>KDYPDNVMTAEMRKIAMAAVLSGMRVNMCASPASSPNVIWAIELEAEGSGSGASQFFKDNCNRTTASLVEGVELTK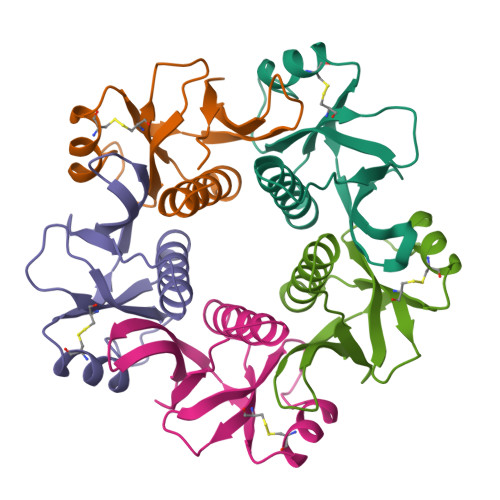YISDINNNTDGMYVVSSTGGVWRISRA[5x]> MTANPTSIHQRLDRRLSGFSLEQPFYTSPEVYALDLQHIFYKQWLYAVPVCQLAKAGSYTTLRVGAYEVVIVRSRDGEVRAFHNSCRHRGSLICKARQGQVAKLVCPYHQWTYELDGKLIWANDMGPDFDASKYGLKPVNLRNLDGLIYICLSDTPPDFQTFAQLARPYLEVHDLKDAKVAFTSTIIEKGNWKLVWENNRECYHCSSNHPALCRSFPLD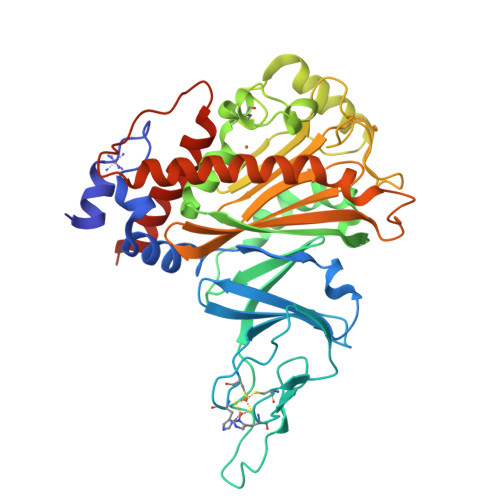PEVAGVQADGGVSKKLQAHFDRCEAAGTPAQFVLAGDGQYRLARMPLQEKALSYTMDGKAAVSRHLGRVAPPDAGTLLMFHYPSTWNHFLPDHSLTFRVMPISPTETEVTTTWLVHKDAVEGVDYDLKRLTEVWIATNDEDREIVETNQQGILSPAYVPGPYSPGQESGVMQFVDWYAASLERALAPRQVAAE> SADKVESLDVDSEAKKLLGLGQKHLVMGDIPAAVNAFQEAASLLGKKYGETANECGEAFFFYGKSLLELARLENKSLQENEEEEIGNLELAWDMLDLAKIIFKRQETKEAQLYAAQAHLKLGEVSVESENYVQAVEEFQSCLNLQEQYLEAHDRLLAETHYQLGLAYGYNSQYDEAVAQFSKSIEVIENRMAVLNEQVKEAEGSSAEYKKEIEELKELLP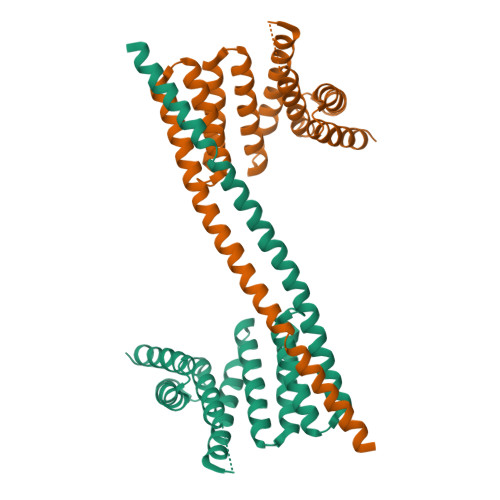EIREKIEDAKESQRSGNVAELALKATLVESST> ASNLKISRMDKTAGSVRGGDEVYLLCDKVQKDDIEVRFYEDDENGWQAFGDFSPTDVHKQYAIVFRTPPYHKMKIERPVTVFLQLKRKRGGDVSDSKQFTYYPV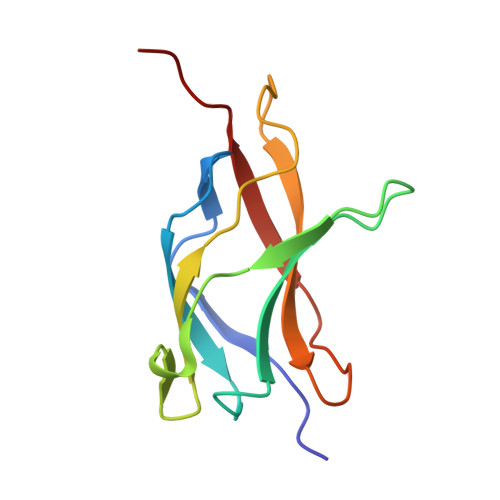VED>[2x]MSLQGIHLSDLSYKHAILKESQYTIKRDVGTTTAVTPSSLQQEITLLCGEILYAKHADYKYAAEIGIQYISTALGSERVQQILRNSGSEVQVVLTRTYSLGKIKNNKGEDLQMLDIHGVEKSWVEEIDKEARKTMATLLKESSGNIPQNQRPSAPDTPIILLCVGALIFTKLASTIEVGLETTVRRANRVLSDAL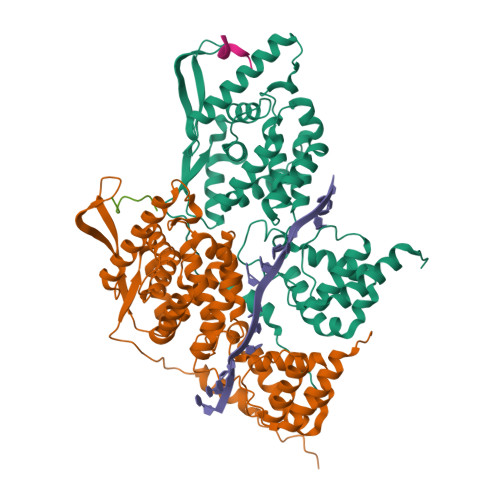KRYPRMDIPKIARSFYDLFEQKVYHRSLFIEYGKALGSSSTGSKAESLFVNIFMQAYGAGQTMLRWGVIARSSNNIMLGHVSVQAELKQVTEVYDLVREMGPESGLLHLRQSPKAGLLSLANCPNFASVVLGNASGLGIIGMYRGRVPNTELFSAAESYAKSLKESNKINFSSLGLTDEEKEAAEHFLNVSDDSQNDYE;>[2x]DIYQLIM>[2x]PR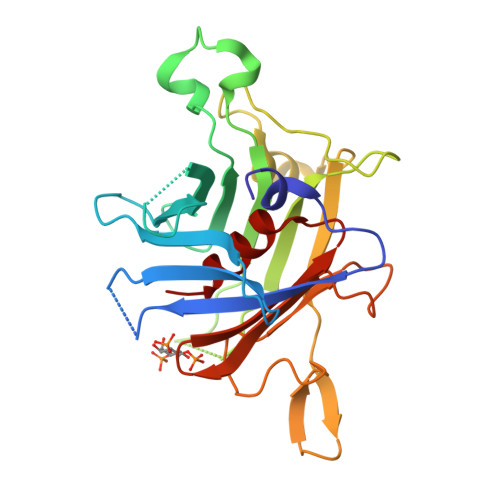EFVLRPAPQGRTVRCRLTRDKKGMDRGMYPSYFLHLDTEKKVFLLAGRKRKRSKTANYLISIDPTNLSRGGENFIGKLRSNLLGNRFTVFDNGQNPQRGYSTNVASLRQELAAVIYETNVLGFRGPRRMTVIIPGMSAENERVPIRPRNASDGLLVRWQNKTLESLIELHNKPPVWNDDSGSYTLNFQGRVTQASVKNFQIVHADDPDYIVLQFGRVAEDAFTLDYRYPLCALQAFAIALSSFD> DLEKGVVLSDLCNFLVSQTIQGWKVYWAGIEFDVTHKGMALLHRLKTNDFAPAWSMTRNLFPHLFQNPNSTIESPLWALRVILAAGIQDQLIDQSLIEPLAGALGLISDWLLTTNTNHFNMRTQRVKE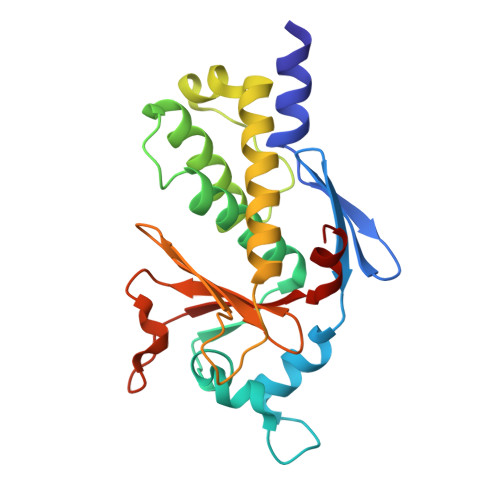QLSLKMLSLIRSNILKFINKLDALHVVNYNGLLSSIEIGTQNHTIIITRTNMGFLVELQEPDKSAMNRMKPGPAKFSLLHESTLKAFT> ENRIQWCAVGKDEKSKCDRWSVVSNGDVECTVVDETKDCIIKIMKGEADAVALDGGLVYTAGVCGLVPVMAERYDDESQCSKTDERPASYFAVAVARKDSNVNWNNLKGKKSCHTAVGRTAGWVIPMGLIHNRTGTCNFDEYFSEGCAPGSPPNSRLCQLCQGSGGIPPEKCVASSHEKYFGYTGALRCLVEKGDVAFIQHSTVEENTGGKNKADWAK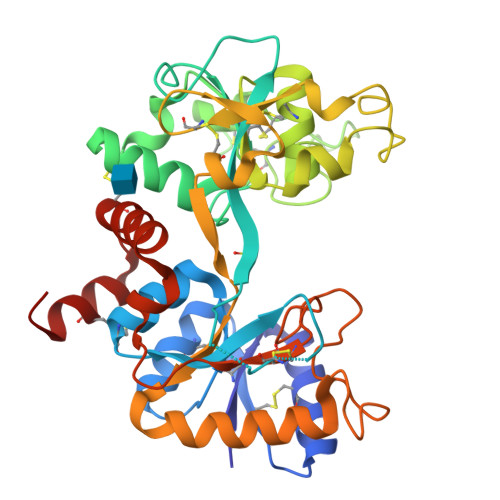NLQMDDFELLCTDGRRANVMDYRECNLAEVPTHAVVVRPEKANKIRDLLERQEKRFGVNGSEKSKFMMFESQNKDLLFKDLTKCLFKVREGTTYKEFLGDKFYTVISSLKTCNPSDILQMCSFLEGK> MWAPPAAIMGDGPTKKVGNQAPLQTQALQTASLRDGPAKRAVWVR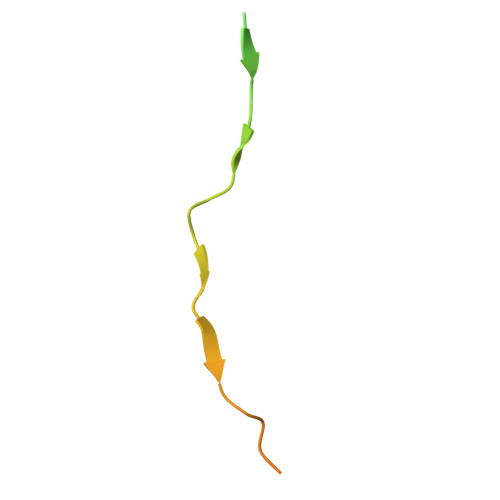HTSSEPQEPTESKAAKERPK>MSGTRASNDRPPGTGGVKRGRLQQEAAATGSRVTVVLGAQWGDEGKGKVVDLLATDADIVSRCQGGNNAGHTVVVDGKEYDFHLLPSGIINTKAVSFIGNGVVIHLPGLFEEAEKNEKKGLKDWEKRLIISDRAHLVFDFHQAVDGLQEVQRQAQEGKNIGTTKKGIGPTYSSKAARTGLRICDLLSDFDEFSARFKNLAHQHQSMFPTLEIDVEGQLKRLKGFAERIRPMVRDGVYFMYEALHGPPKKVLVEGANAALLDIDFGTYPFVTSSNCTVGGVCTGLGIPPQNIGDVYGVVK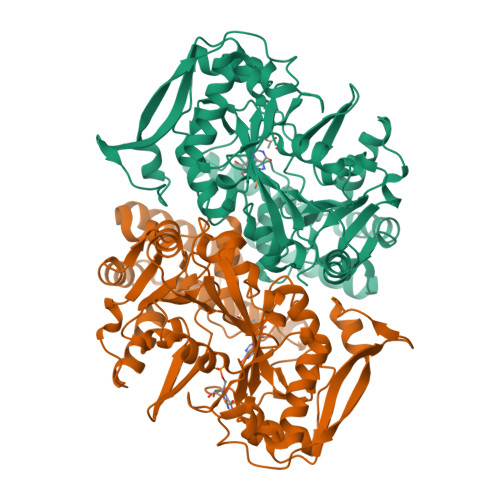AYTTRVGIGAFPTEQINEIGDLLQNRGHEWGVTTGRKRRCGWLDLMILRYAHMVNGFTALALTKLDILDVLSEIKVGISYKLNGKRIPYFPANQEILQKVEVEYETLPGWKADTTGARKWEDLPPQAQSYVRFVENHMGVAVKWVGVGKSRESMIQLF[2x]>[2x]MKLSRISAINWNKIQDDKDLEVWNRLTSNFWLPEKVPLSNDIPAWQTLSAAEQQLTIRVFTGLTLLDTIQNIAGAPSLMADAITPHEEAVLSNISFMEAVHARSYSSIFSTLCQTKEVDAAYAWSEENPPLQRKAQIILAHYVSDEPLKKKIASVFLESFLFYSGFWLPMYFSSRGKLTNTADLIRLIIRDEAVHGYYIGYKYQIALQKLSAIEREE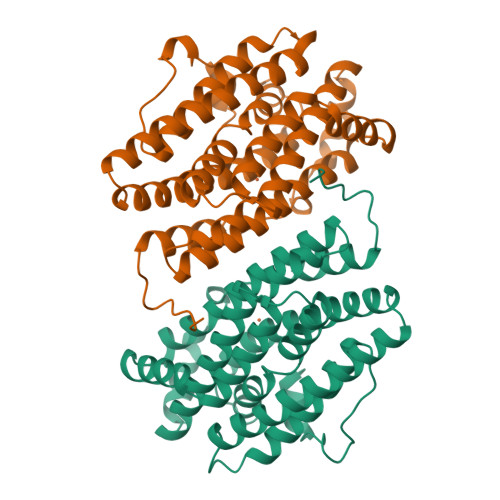LKLFALDLLMELYDNEIRYTEALYAETGWVNDVKAFLCYNANKALMNLGYEALFPPEMADVNPAILAALSPNADENHDFFSGSGSSYVMGKTVETEDEDWNF>[2x]EAEAAGLNTAAKAKGLKYFGSATDNPELTDSAYVAQLSNTDDFGQITPGNSMKWDATEPSQNSFSFANGDAVVNLANKNGQLMRCHTLVWHSQLPNWVSSGSWTNATLLAAMKNHITNVVTHYKGKCYAWD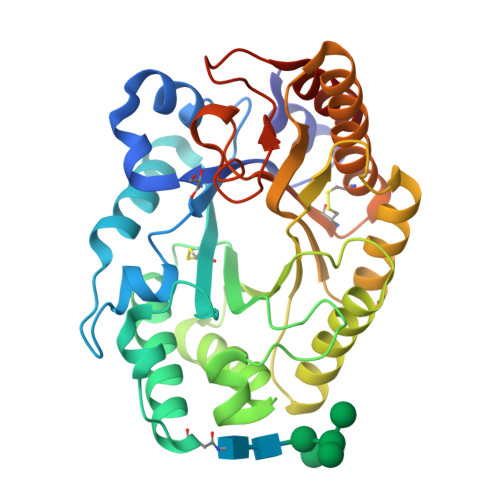VVNEALNEDGTFRNSVFYQIIGPAYIPIAFATAAAADPDVKLYYNDYSIEYSGAKATAAQNIVKMIKAYGAKIDGVGLQAHFIVGSTPSQSDLTTVLKGYTALGVEVAYTELDIRMQLPSTAAKLAQQSTDFQGVAAACVSTTGCVGVTIWDWTDKYSWVPSVFQGYGAPLPWDENYVKKPAYDGLMAGLGASGSGTT>MEKPTPLINSSMLGQYVGQTVRIVGKVHKVTGNTLLMQTSDLGNVEIAMTPDSDVSSSTFVEVTGKVSDAGSSFQANQIREFTTVDCGHDVDLTLVENVVQISAAFPNLFSDST[2x];>GKKAGNNTLRPVTIRQILNAEQPHPDAEFILDGAELGQLTFVAVVRNISRNATNVAYSVEDGTGQIEVRQWLDSSSDDSSKASEIRNNVYVRVLGTLKSFQNRRSISSGHMRPVIDYNEVMFHRLEAVHAHLQVTR[2x];>[2x]MPIYPIEGLSPYQNRWTIKARVTSKSDIRHWSNQRGEGKLFSVNLLDDSGEIKATGFNDAVDRFYPLLQENHVYLISKARVNIAKKQFSNLQNEYEITFENSTEIEECTDATDVPEVKYEFVRINELESVEANQQCDVIGILDSYGELSEIVSKASQRPVQKRELTLVDQGNRSVKLTLWGKTAETFPTNAGVDEKPVLAFKGVKVGDFGGRSLSMFSSSTMLINPDITESHVLRGWYDNDGAHAQFQPYTNGGVGGGAMGGGGAGANMAERRTIVQVKDENLGMSEKPDYFNVRATVVYIKQENLYYTACASEGCNKKVNLDHENNWRCEKCDRSYATPEYRYILSTNVADATGQMWLSGFNEDATQLIGMSAGELHKLREESESEFSAALHRAANRMYMFNCRAKM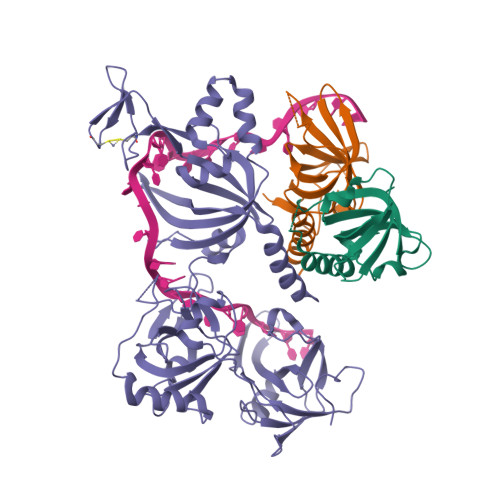DTFNDTARVRYTISRAAPVDFAKAGMELVDAIRAYM>[4x]GAMGTEKVLQICPKDMRADICVHLNRKVFKEHPAFRLASDGCLRALAMEFQTVHCAPGDLIYHAGESVDSLCFVVSGSLEVIQDDEVVAILGKGDVFGDVFWKEATLAQSCANVRALTYCDLHVIKRDALQKVLEFYTAFSHSFSRNLILTYNLRKRIVFRKISDVKRE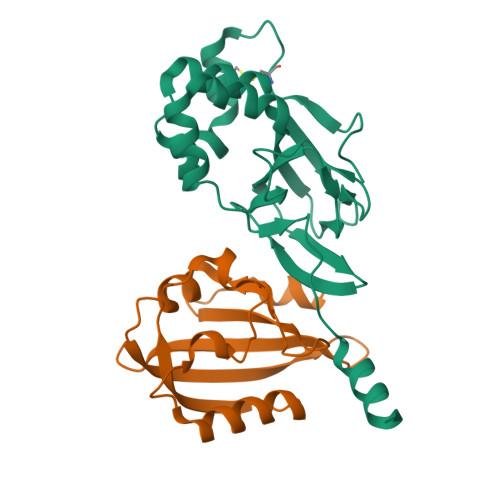EEERMKRK;>GAMGRRGLVAPQNTFLENIVRRSNDTNFVLGNAQIVDWPIVYSNDGFCKLSGYHRAEVMQKSSACSFMYGELTDKDTVEKVRQTFENYEMNSFEILMYKKNRTPVWFFVKIAPIRNEQDKVVLFLCTFSDITAF[4x]>AECRFVGLTNLGATCYLASTIQQLYMIPEARQAVFTAKYSEDMKHKTTLLELQKMFTYLMESECKAYNPRPFCKTYTMDKQPLNTGEQKDMTEFFTDLITKIEEMSPELKNTVKSLFGGVITNNVVSLDCEHVSQTAEEFYTVRCQVADMKNIYESLDEVTIKDTLEGDNMYTCSHCGKKVRAEKRACFKKLPRILSFNTMRYTFNMVTMMKEKVNTHFSFPLRLDMTPYTEDFLMGKSERKEGFKEVSDHSKDSESYEYDLIGVTVHTGTADGGHYYSFIRDIVNPHAYKNNKWYLFNDAEVKPFDSAQLASECFGGEMTTKTYDSVTDKF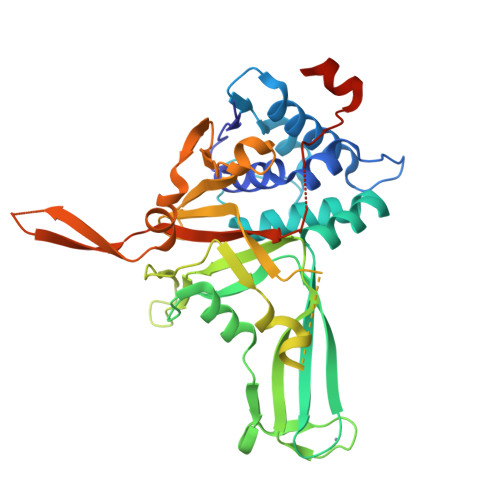MDFSFEKTHSAYMLFYKRMEPEEENGREYKFDVSSELLEWIWHDNMQFLQDK[2x]> SVEWE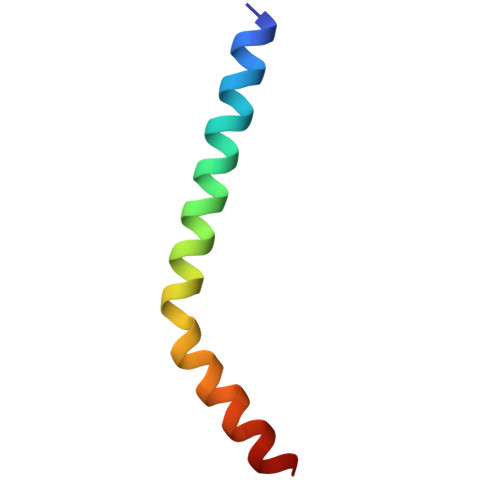NCVSVIEAAILKHKYKQKVNKNIPSLLRVQAHIRKKMV For the levan utilisation system, the cell surface components are Bt1760 (a GH32 endo-levanase), Bt1761 (a surface glycan-binding protein; SGBP), Bt1762 (SusD) and Bt1763 (SusC)15,19,24. SusC proteins are unique among TBDTs in that they are tightly associated with a SusD substrate-binding lipoprotein15–17. Recently, we showed that SusCD complexes mediate substrate uptake via a “pedal bin” mechanism. The SusC transporter forms the barrel of the bin, while SusD sits on top of the barrel, opening and closing like a lid to facilitate substrate binding.

Next, we obtained a structure without a substrate using a protein preparation that did not suffer from proteolysis. Interestingly, while this structure is very similar to that reported earlier, density for the plug domain is poor but clearly present, suggesting mobility or different conformations of the plug within the barrel. While there is no density supporting this notion, it is also possible that the plug has been ejected from some of the Bt1763 barrels in the crystal. Consistent with the relatively high solvent content of the crystals (~63%), there are large spaces underneath the barrels that could contain ejected and mobile plug domains. Superposition of the crystal structures of plug-less and complete transporters indeed show non-uniform displacements of up to ~2–2.5 Å for Cα atoms of barrel wall residues, which is substantially more than the coordinate errors of the structures (~0.5 Å), showing that the barrels have subtly different shapes. The very similar crystal structures of Bt1762-63 in the absence and presence of FOS appear at odds with the dynamics proposed in the pedal bin transport model, but are likely explained by the fact that crystallisation selects for compact, stable states.

> MKKIIYIATIGITLLTTSCDDFLDRQVPQGIVTGDQIASPEYVDNLVISAYAIWATGDDINSSFSLWNYDVRSDDCYKGGSGTEDGGVFNALEISKGINTTDWNINDIWKRLYQCITRANTALQSLDQMDEKTYPLKNQRIAEMRFLRGHAHFMLKQLFKKIVIVNDENMEPDAYNELSNTTYTNDEQWQKIADDFQFAYDNLPEVQIEKGRPAQAAAAAYLAKTYLYKAYRQDGADNALTGINEEDLKQVVKYTDPLIMAKGGYGLETDYSMNFLPQYENGAESVWAIQYSINDGTYNGNLNWGMGLTTPQILGCCDFHKPSQNLVNAFKTDSQGKPLFSTYDNENYEVATDNVDPRLFHTVGMPGFPYKYNEGYIIQKNDDWSRSKGLYGYYVSLKENVDPDCDCLKKGSYWASSLNHIVIRYADVLLMRAEALIQLNDGRITDAISLINEVRSRAAGSTMLIFNYKEDYGVNFKVTPYDLKAYAQDEAMKMLKWERRVEFGMESSRFFDLVRWGEAKDVINAYYVTEASRCSIYKNAGFTENKNEYLPVPFEQISASNGNYTQNFGWAAAAHHHHHH;> MPGIMKNKKLLCSVCFLFAFMSALWGQNITVKGNVTSKTDGQPIIGASVVETTATTNGTITDFDGNFTLSVPVNSTLKITYIGYKPVTVKAAAIVNVLLEEDTQMVDEVVVTGYTTQRKADLTGAVSVVKVDEIQKQGENNPVKALQGRVPGMNITADGNPSGSATVRIRGIGTLNNNDPLYIIDGVPTKAGMHELNGNDIESIQVLKDAASASIYGSRAANGVIIITTKQGKKGQIKINFDASVSASMYQSKMNVLNTEQYGRAMWQAYVNDGENPNGNALGYAYNWGYNADGNPVLYGMTLSKYLDSKNTMPVADTDWFDEITRTGVIQQYNLSVSNGSEKGSSFFSLGYYKNLGVIKDTDFDRFSARMNSDYKLIDDILTIGQHFTLNRTSEVQAPGGIIETALDIPSAIPVYASDGSWGGPVGGWPDRRNPRAVLEYNKDNRYTYWRMFGDAYVNLTPFKGFNLRSTFGLDYANKQARYFTYPYQEGTQTNNGKSAVEAKQEHWTKWMWNAIATYQLEVGKHRGDVMIGMELNREDDSHFSGYKEDFSILTPDYMWPDAGSGTAQAYGAGEGYSLVSFFGKMNYSYADRYLLSLTLRRDGSSRFGKNHRYATFPSVSLGWRITQENFMKELTWLDDLKLRASWGQTGNQEISNLARYTIYAPNYGTTDSFGGQSYGTAYDITGSNGGGVLPSGFKRNQIGNDNIKWETTTQTNVGIDFSLFKQSLYGSLEYYYKKATDILTEMAGVGVLGEGGSRWINSGAMKNQGFEFNLGYRNKTAFGLTYDLNGNISTYRNEILELPETVAANGKFGGNGVKSVVGHTYGAQVGYIADGIFKSQDEVDNHATQEGAAVGRIRYRDIDHNGVIDERDQNWIYDPTPSFSYGLNIYLEYKNFDLTMFWQGVQGVDIISDVKKKSDFWSASNVGFLNKGTRLLNAWSPTNPNSDIPALTRSDTNNEQRVSTYFVENGSFLKLRNIQLGYTVPAVISKKMRMDRLRFYCSAQNLLTIKSKNFTGEDPENPNFSYPIPVNITFGLNIGF> MQYIIGIGTNIGFTIENIHLAITALESQQNIRIIRKASLYSSKAVLKEDAPKEWDIRFLNTAVKISSSLKPDELLVLLKDIELKIGRDLNAPAWSPRVIDLDILAAEDLILETDKLTIPHKELINRSFALAPLLELSKGWHHPKYVEWDLNIRLKELGEIVKLKQTLANTIRMGIVNLSNQSFSDGNFDDNQRKLNLDELIQSGAEIIDIGAESTKPDAKPISIEEEFNKLDEFLEYFKSQLANLIYKPLVSIDTRKLEVMQKILAKHHDIIWMINDVECNNIEQKAQLIAKYNKKYVIIHNLGITDRNQYLDKENAIDNVCDYIEQKKQILLKHGIAQQNIYFDIGFGFGKKSDTARYLLENIIEIKRRLELKALVGHSRKPSVL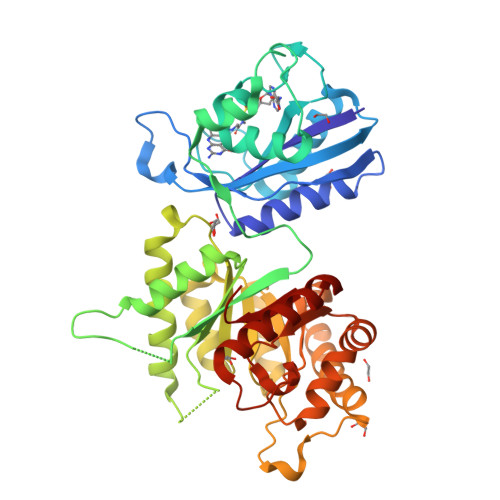GLAKDSNLATLDRATRELSRKLEKLDIDIIRVHKI> MDATALERDAVQFARLAVQRDHEGRYSEAVFYYKEAAQALIYAEMAGSSLENIQEKITEYLERVQALHSAVQSKSADPLKSKHQLDLERAHFLVTQAFDEDEKENVEDAIELYTEAVDLCLKTSYETADKVLQNKLKQLA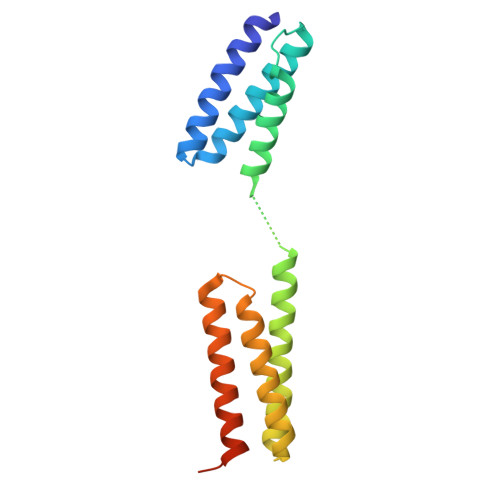RQALDRAEALSEPLTKPVGKISSTS>[2x]AANDNNVEWNGLFHDQGPLFDNAPEPTSTQSVTLKLRTFKGDITSANIKYWDTADNAFHWVPMVWDSNDPTGTFDYWKGTIPASPSIKY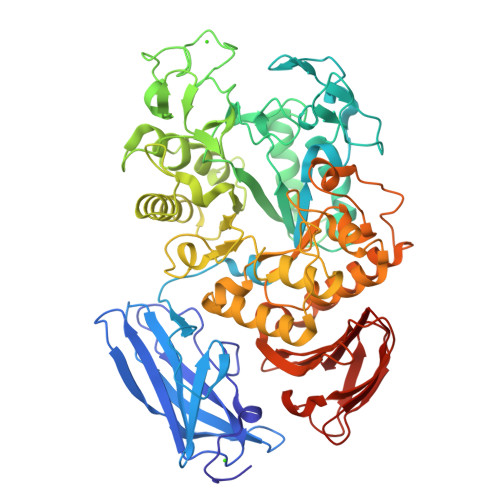YRFQINDGTSTAWYNGNGPSSTEPNADDFYIIPNFKTPDWLKNGVMYQIFPDRFYNGDSSNDVQTGSYTYNGTPTEKKAWGSSVYADPGYDNSLVFFGGDLAGIDQKLGYIKKTLGANILYLNPIFKAPTNHKYDTQDYMAVDPAFGDNSTLQTLINDIHSTANGPKGYLILDGVFNHTGDSHPWFDKYNNFSSQGAYESQSSPWYNYYTFYTWPDSYASFLGFNSLPKLNYGNSGSAVRGVIYNNSNSVAKTYLNPPYSVDGWRLDAAQYVDANGNNGSDVTNHQIWSEFRNAVKGVNSNAAIIGEYWGNANPWTAQGNQWDAATNFDGFTQPVSEWITGKDYQNNSASISTTQFDSWLRGTRANYPTNVQQSMMNFLSNHDITRFATRSGGDLWKTYLALIFQMTYVGTPTIYYGDEYGMQGGADPDNRRSFDWSQATPSNSAVALTQKLITIRNQYPALRTGSFMTLITDDTNKIYSYGRFDNVNRIAVVLNNDSVSHTVNVPVWQLSMPNGSTVTDKITGHSYTVQNGMVTVAVDGHYGAVLAQ> MASMTGGQQMGRGSMQNPSV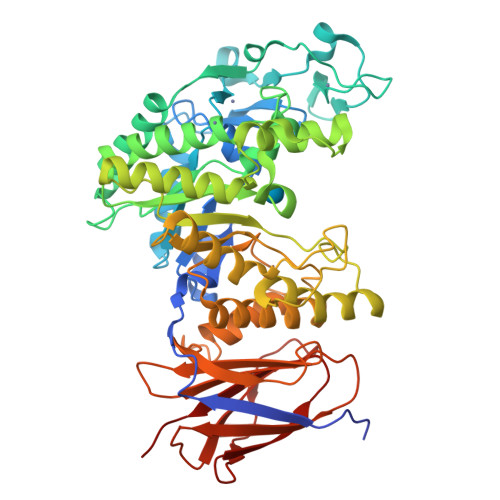TISVNANAGRHPINPAVYGLAYATTATLADLNVPLHRYGGNNTSRYNWQLNADNRGADWYFESIGEASSVAGERGDTFIANSQAAGAQAMITIPTIGWVARLGANRSKLASFSIAKYGAQSGNDWQWFPDAGNGVLTSGQNVTGNNPNDANTLVDSTFQQGWAQHLVSQWGTAAGGGLRYYILDNEPSIWFSTHRDVHPVGPTMDEIRDKMLDYGAKIKTVDPSALIVGPEEWGWSGYTLSGYDQQYGGLHGWSFMPDRNNHGGWDYLPWLLDQLRQNNLSTGRRLLDVFSVHYYPQGGEFGNDTSSAMQLRRNRSTRSLWDPNYIDETWINDKVQLIPRLKNWVSTYYPGTLTAITEYNWGAESHINGATTQADILGIFGREGLDMAARWTTPDTATPTYKAIKMYRNYDGNKSAFGDTSVTATAPNPDNVSAFAAVRSSDGALTVMVINKYLSGNTPATINLSNFTAQAQAQVWQLTAANTINHLSNVSLSGSSLSLTLPAQSVTLLVIPAST>KPAPSTIFSPEKALGLLLSLKLSKWQYITLRETTIREGSKEIYPSYYKVQKAKLQCYPPKAFVAVTDSSAKIALQALLDLTVNRIFETIRSPDAIQNKQLILISKWGFDGASNQSRYKQNIESGQGDSSIFMTSLVPLKLTADGDTVWVNPKPCSPMYCRPVQFSFVKETKDVVINEKTAMDDEIEALVPSKCQGHEISHKLMMTMIDGKICTYLSEAKSNAACYLCLAKPTEMSKLDVIASKTISSGVYEFGLSTLHARINVMECLLHIAYRLDFKKWSARGEGHQELLHSRKKLIQDRFKDDLNLLIDIVKQGSGTTNDGNTARRFFEFPDKTAAITGLDEDLIRRFSVILQAITSGEIIDVPKFKEYARTTAEKYVELYDWYYMSSTVHKLLIHGGDIIAENAIVPIGSLSEEASEARNKDFRRFREHHSRKKSRQASNEDILNMLIISSDPLISFTRPKLDAHKRQTYFKETVELLQLQDQEAPTEFHHHHHH[2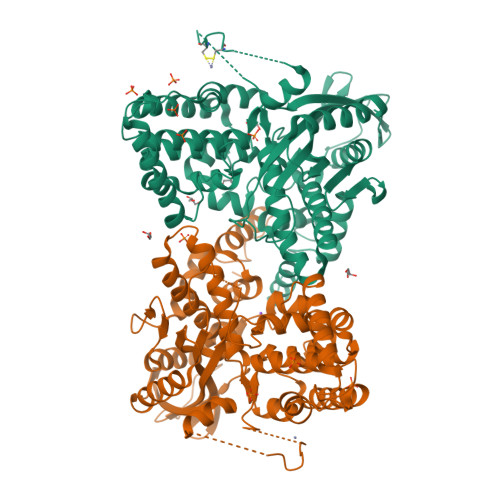x]4,4'-(thiophene-2,5-diyl)dibenzoic acid | C18 H12 O4 S | 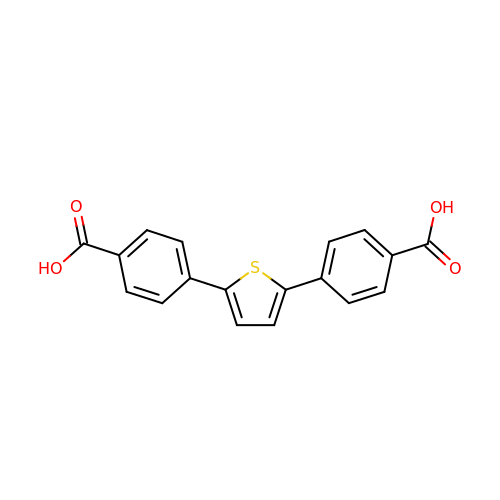XUZWFMDZGVUJPF-UHFFFAOYSA-N>MSEIQTAHTHSAPLVGVLMGSSSDWDVMKHAVAILQEFGVPYEAKVVSAHRMPDEMFDYAEKARERGLRAIIAGAGGAAHLPGMLAAKTTVPVLGVPVASKYLKGVDSLHSIVQMPKGVPVATFAIGEAGAANA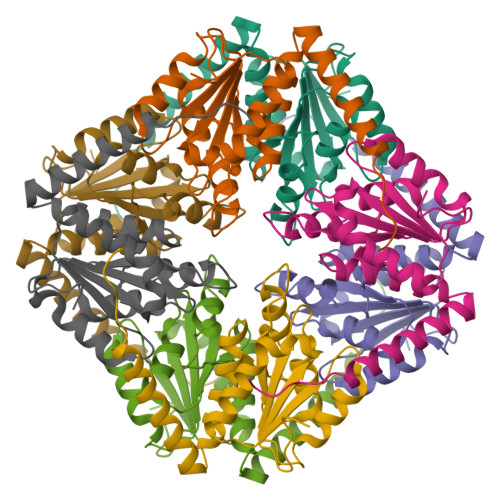ALFAVSILSGNSVDYANRLAAFRVRQNEAAHAMVLPPLE[4x]RNR is an essential enzyme found in almost every organism that converts ribonucleotides to deoxyribonucleotides. The first-identified and most-studied class of RNRs, the class Ia RNRs, uses a diiron-oxo center to generate a stable tyrosyl radical in the radical-generating β subunit that travels >30 Å to the active site in the catalytic α subunit to remove the 2′-hydroxyl group from the ribonucleotide diphosphate substrate. In order to respond to the deoxyribonucleotide needs of the organism, class Ia RNRs have two allosteric sites in addition to the catalytic site: the specificity site, which determines which of the four ribonucleotide substrates is bound in the active site; and the activity site, which acts as a general on/off switch for the enzyme. When dATP is bound in the activity site, class Ia RNR enzymes have been shown to form ring-shaped structures that physically prevent radical transfer between the β and α subunits; when ATP displaces dATP, the β and α subunits can come together to form an active α2β2 complex.

The 4.3 Å resolution structure of Neisseria gonorrhoeae class Ia RNR in the inactive α4β4 oligomeric state solved using the chameleon with a fast dispense-to-plunge time yields molecular information regarding similarities and differences to the well studied Escherichia coli class Ia RNR α4β4 ring. Here, we were able to generate a structure of the N. gonorrhoeae inactive RNR complex resolved to 0.744x the Nyquist limit (4.3 Å resolution at 1.5998 Å/pixel) through the use of the blot-free chameleon with a fast (54 ms) dispense-to-plunge time but not through a traditional blotting-based plunging technique (which produced a 5.6 Å resolution structure). First, we confirmed that in the presence of activity effector dATP, the N. gonorrhoeae class Ia RNR forms a protein complex similar in structure and subunit composition to the well studied E. coli class Ia RNR. In particular, when dATP is bound to the activity sites within the N-terminal regions (i.e., cone domains) of either the E. coli or N. gonorrhoeae α subunits, each α subunit interacts with a β subunit, forming four α/β interfaces and an α4β4 ring-shaped structure. Within the N. gonorrhoeae α/β interface, there is density for residues homologous to the E. coli class Ia RNR interface residues, indicating close similarity between the two structures in this region; additionally, a similar amount of solvent-accessible surface area (495 Å2 and 575 Å2 for N. gonorrhoeae and E. coli, respectively) is buried in the α/β interface upon formation of the α4β4 structure. Density for both residues S41 and H25, which have recently been identified as important residues for organism viability and drug resistance, are visible in the α/β interface region, suggesting that the compounds may act on the α/β interface region.

>[4x]MGHHHHHHENLYFQMNTPTDLKVTKRDGRLEAIDLDKIHRVVTWAAEGLENVSVSQVELKSHIQFYNGIRTDDIHETIIKAAADLISEDTPDYQYLAARLAIFHLRKIAYGEYEPPHLYNHVKKLTDAGKYDRHILEDYSREEFDELNAYIDHERDMSFSYAAVKQLEGKYLVQNRVTRQIYETPQFLYVLVAMCLFSKYPKEARLDYVKRFYDAVSTFKVSLPTPIMSGVRTPTRQFSSCVLIECDDSLDSINATTSAIVKYVSQRAGIGINAGRIRGLDSEIRGGEARHTGCIPFFKMFQAAVKSCSQGGVRGGAATLFYPLWHIEAESLLVLKNNRGVEDNRIRQLDYGVQINRLLYTRLIKGGNITLFSPNEVSGLYEAFFADQDEFERLYTKYEQDPNIRKRIIPAADLFSTLMQERAGTGRIYIQNVDHCNTHSPFDPRVAPVHQSNLCMEIALPTKPLDNINDPDGEIALCTLSAFNLGALNSLDELEGLADLTVRALDALLDYQGYPVEAARTSTMDRRSLGIGVINYAYYLAKNGVRYSDGSALGLTHRTFEAIQYYLLKASANLAKEYGACTLFNQTVYSQGKLPIDTYKKDLDAVCGEPLHYDWESLRADIVKYGLRNSTLTALMPSETSSQIANATNGIEPPRGLVTVKASKDGILKQVVPEFETLKNAYETLWQLPGNEGYLKLVGVMQKFVDQAISANTAYDPGKFEGNKVSMKQMLKDLLTAYKYGVKTLYYHNTRDGADDTQTDIQDDGCAGGACKI;>MGHHHHHHENLYFQMSYSTFPKTKNDALKEPMFFGQPVNVARYDQQKYEVFEKLIEKQLSFFWRPEEIDVSRDRIDYANLPEHEKHIFISNLKYQTLLDSIQGRSPNVALLPLVSIPELETWVETWSFSETIHSRSYTHIIRNIVNDPSVVFDDIVENEYITARAEDIACYYDDLIEYTQYYNLLGEGVHNVGGKPVTVSLRGLKKKLYLCLMCVNVLEAIRFYVSFACSFAFAERELMEGNAKIIKDIARDEALHLTGTQHMLNLMRSGVDDPEMAEIAAELQDECFQLFKKAAEQEKEWAAYLFKDGSMIGLNKEILSQYVEYITNLRMQAVGLPAGFEGANQNPIPWINAWLSSDNVQVAPQEVEISSYLIGQIDSEVNTDDLGDFEL[4x]(3-ENDO)-8-METHYL-8-AZABICYCLO[3.2.1]OCT-3-YL 1H-INDOLE-3-CARBOXYLATE | 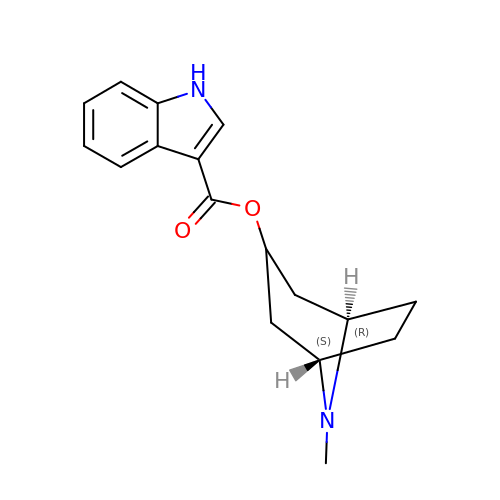C17 H20 N2 O2 | ZNRGQMMCGHDTEI-ITGUQSILSA-N> LDNVATYAGQFNQD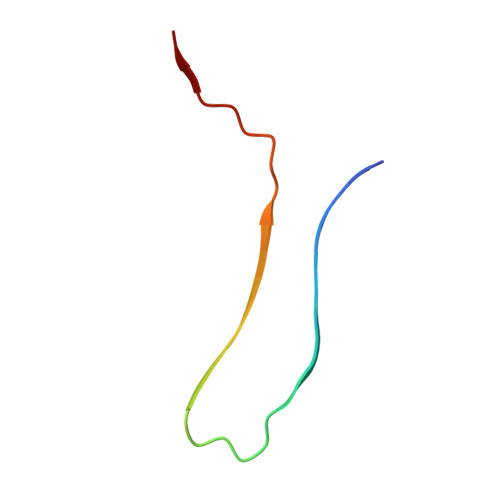YLSGMAANMSGTFGGANMPNLY> GDSLSIHQLAAQGELDQLKEHLRKGDNLVNKPDERGFTPLIWA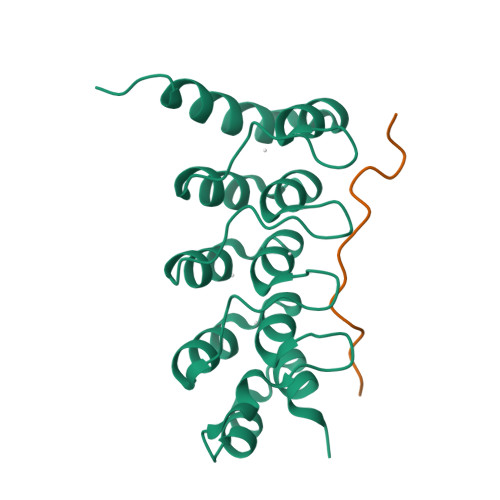SAFGEIETVRFLLEWGADPHILAKERESALSLASTGGYTDIVGLLLERDVDINIYDWNGGTPLLYAVHGNHVKCVEALLARGADLTTEADSGYTPMDLAVALGYRKVQQVIENHILKLFQSNLVPADPE;> LPLYTSPSLPNITLGLP>ATVPLPAEGEIGLVHIGALTLENGTVLPDVTIAVQRWGELAPDRGNVVMVLHALTGDSHVTGPAGDGHPTAGWWDGVAGPGAPIDTDHWCAIATNVLGGCRGSTGPGSLAPDGKPWGSRFPQITIRDQVAADRAALAALGITEVAAVVGGSMGGARALEWLVTHPDDVRAGLVLAVGARATADQIGTQSTQVAAIKADPDWQGGDYHGTGRAPTEGMEIARRFAHLTYRGEEELDDRFANTPQDDEDPLTGGRYAVQSYLEYQGGKLARRFDPGTYVVLSDALSSHDVGRG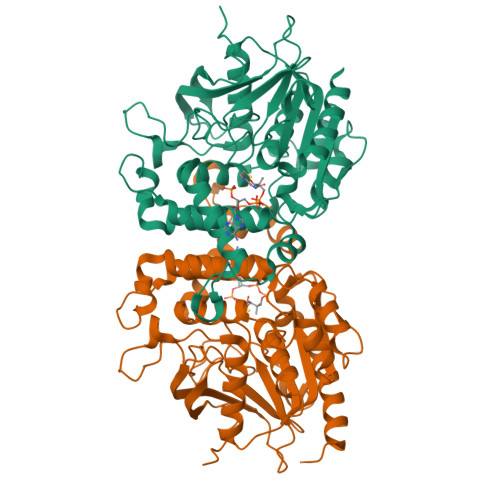RGGVEAALRSCPVPVVVGGITSDRLYPIRLQQELAELLPGCQGLDVVDSIYGHDGFLVETELVGKLIRRTLELAQRLEHHHHH[2x]N-{6-[2-(methylsulfanyl)pyrimidin-4-yl]-1,3-benzothiazol-2-yl}acetamide | C14 H12 N4 O S2 | 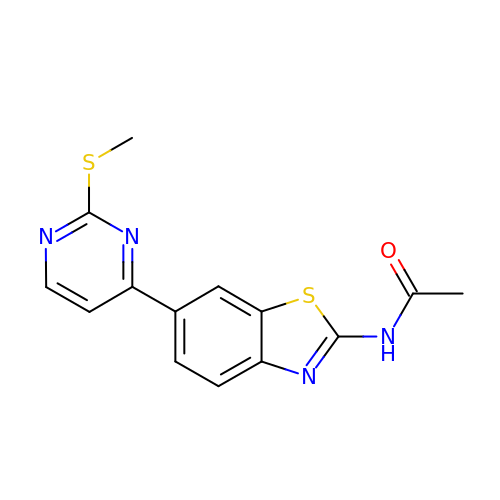UJBQBHAEDABZIB-UHFFFAOYSA-N> GSGAMERVLKVFHYFENSSEPTTWASIIRHGDATDVRGIIQKIVDCHKVKNVACYGLRLSHLQSEEVHWLHLDMGVSNVREKFELAHPPEEWKYELRIRYLPKGFLNQFTEDKPTLNFFYQQVKNDYMLEIADQVDQEIALKLGCLEIRRSYGEMRGNALEKKSNYEVLEKDVGLRRFFPKSLLDSVKAKTLRKLIQQTFRQFANLNREESILKFFEILSPVYRFDKECFKCALGSSWIISVELAIGPEEGISYLTDKGANPTHLADFNQVQTIQYSNSEDKDRKGMLQLKIAGAPEPLTVTAPSLTIAENMADLIDGYCRLVNGATQSFIIRPQKEGERALPSIPKLANNEKQGVRSHTVSVSETDDYAE;> STRDYEI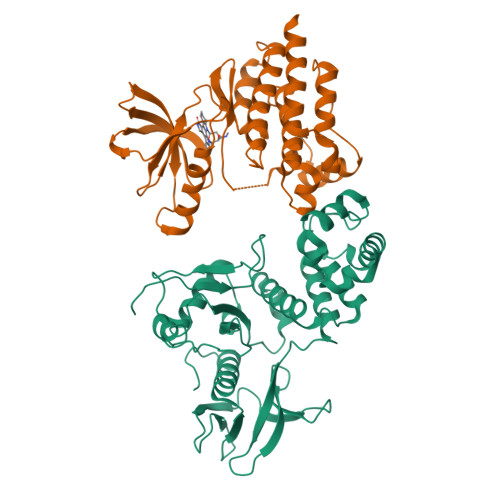QRERIELGRCIGEGQFGDVHQGIYMSPENPALAVAIKTCKNCTSDSVREKFLQEALTMRQFDHPHIVKLIGVITENPVWIIMELCTLGELRSFLQVRKYSLDLASLILYAYQLSTALAYLESKRFVHRDIAARNVLVSSNDCVKLGDFGLSRYMEDSTYYKASKGKLPIKWMAPESINFRRFTSASDVWMFGVCMWEILMHGVKPFQGVKNNDVIGRIENGERLPMPPNCPPTLYSLMTKCWAYDPSRRPRFTELKAQLSTILEEEKLQ> APKCIECHINIEMDPVLHDVFKLQVCKQCSKEHPEKYALLTKTECKEDYFLTDPELNDEDLFHRLEKPNPHSGTFARMQLFVRCEVEAFAFKKWGGEEGLDEEWQRREE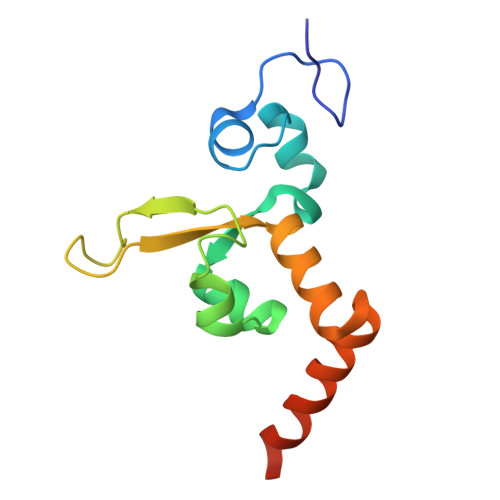GKAHRREKKY> TKRFYVKDHRNKAMINLHIQKDNPKIVHAFDMEDLGDKAVYCRCWRSKKFPFCDGAHTKHNEET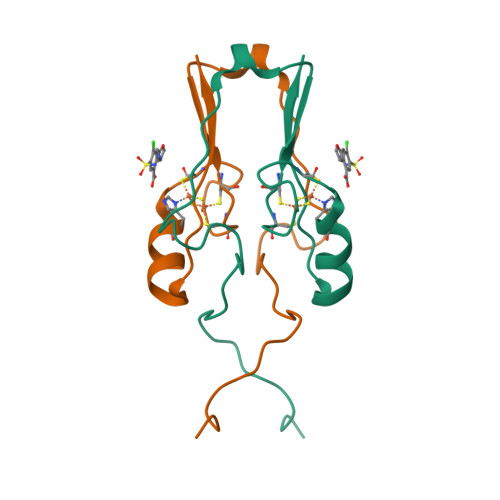GDNVGPLIIKKKET2',5'-dideoxy-5'-(tritylamino)uridine | C28 H27 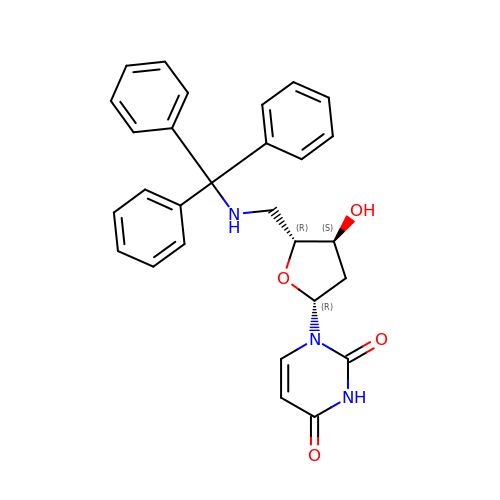N3 O4 | TUZNCXRMWDUVNX-BFLUCZKCSA-N>[2x]MGSSHHHHHHSQDPENLYFQGSAANADFELFRVFLEKTCGIVLGSNKQYLVSSRLNKLMEQQGIKSLGELVQRIQ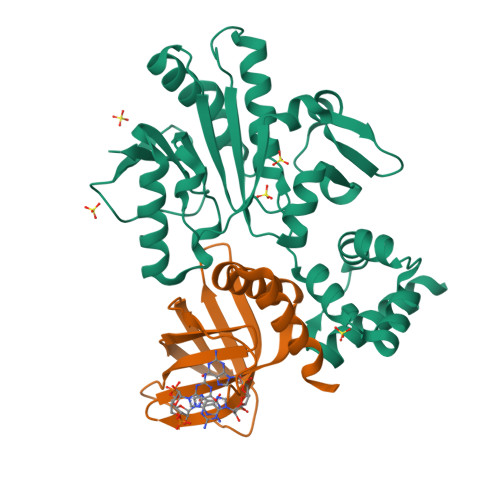TQRGGLREMVVDAMTTNETLWFRDTYPFEVLKQRVLPELIKANGGQRLRIWSAACSSGQEPYSLSMAIDEFEKTNLGQLKAGVQIVATDLSGSMLTAAKAGEYDTLAMGRGLSPERLQRYFDAKGPGRWAVKPAIRSRVEFRALNLLDSYASLGKFDMVFCRNVLIYFSAEVKRDILLRIHGTLKPGGYLFLGASEALNNLPDHYQMVQCSPGIIYRAK;>[2x]MGSSHHHHHHSQDPENLYFQGSDQHDERRRFHRIAFDADSEILQGERRWEVLLHDVSLHGILVGQPQDWNGDPQRPFEARLYLGLDVLIRMEISLAWARDGLLGFECQHIDLDSISHLRRLVELNLGDEELLERELALLVSAHDD>[12x]SPLERRLKEHIIGQEGAINTVASAIRRKENGWYDEEHPLVFLFLGSSGIGKTELAKQVARYMHKDIKKGFIRMDMSEFQEKHEVAKFIGSPPGYVGHDEGGQLTKQLKQSPSAVVLFDEVEKAHPDVLTVMLQLFDEGRLTDGKGKTIECKDAIFIMTSNAA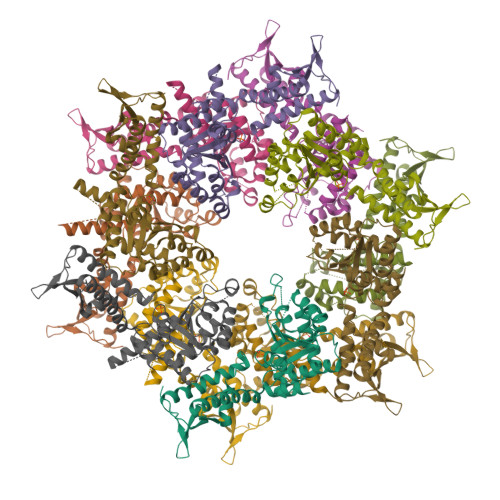SDEIAQHALQLRQEAQEQSRRRLAENLDDVQKSENITISNTFKEQVIRPILKAHFRRDEFLGRINEIVYFLPFCHSELLQLVSRELHYWAKKAKQRHNITLLWERPVLELLVKGYNLHYGARSIKHEVERRVVNQLAAAFEQELLPKGCTLRLTVDRDSQHTDGAPVLRLELLQEDKTSRKLEIQPPLNPQDTAHTPRKH> IVGGYNCKDGEVPWQALLINEENEGFCGGTILSEFYILTAAHCLYQAKRFKVRVGDRNTE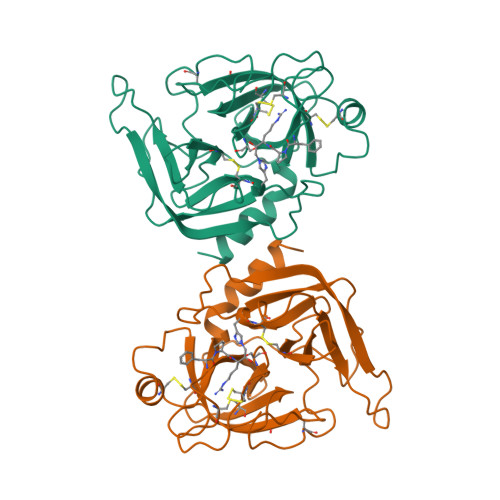QEEGGEAVHEVEVVIKHNRFTKETYDFDIAVLRLKTPITFRMNVAPASLPTAPPATGTKCLISGWGNTASSGADYPDELQCLDAPVLSQAKCEASYPGKITSNMFCVGFLEGGKDSCQGDSGGPVVCNGQLQGVVSWGDGCAQKNKPGVYTKVYNYVKWIKNTIAANS> MEQIAQQQPQTLCIKHLAKNYSKRWVVKDVSFEMQSGQIVGLLGPNGAGKTTSFYMVVGLVRMDKGEIHLDNLDLSDLAMHERARKGIGYLPQEASIFRKLTIAENIMAILETRKDLNKQQRQQRLQELLNDFKITHIKDSLGMSVSGGERRRAEIARALAADPKFMLLDEPFAGVDPISVGDIKDIIRNLKDRGIGVLITDHNVRETLAICEHAYIVSEGAVIAEG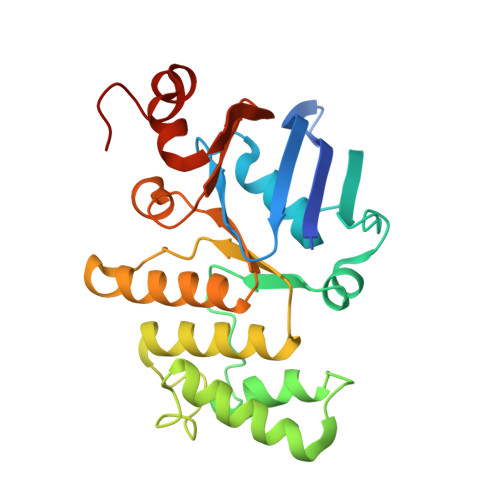SPQDILENEQVRKVYLGDDFTV>MSGSMKEEIKRLAEELKEKTKNEEIKRLAEEAAELAERSDDPEVLEVVKKALEEALKSKNEEKIELLLLVAVLVAEAGSVDAVEEKLEIALLALKLAEESKDPRIIRGALRAAIAALRSDDPLALKTVKEALERARASKDERLIRAILAAAYAFALLAVAGASAERLKEAEAIVKELIAAAEKGASPQELVLLVIEMMVKGMGVTMETHRSGNEVKVVIKGLHESQQEVLLEAVLFAAELMGVRVRIRFKGDTVTIVVREGSG[2x];>MSGEEAVRRRFEELLREALAFRERTGGRRETLEHAVRLARELAEFAASHPEFNRQEAVLLAIELMVRAMGVTMETHRSGNEVKVVIKGLNIDEQVALYRAVRETSKIMGVETEIEVEGDTQTIVVREGSG[2x]

Several natural systems exhibit ‘facilitated dissociation’, in which an effector (E) can bind to a target–host (TH) complex to form an excited ternary complex (THE)20–26 from which the target dissociates quickly. We set out to design protein systems that undergo facilitated dissociation. We use a switchable target binder (host) and a flexible effector that can rapidly bind to and switch the target–host complex to induce a large steric clash with the target, forming a strained excited ternary complex. We show here that by explicitly considering excited intermediate states when designing coupled protein systems, a broad range of facilitated dissociation systems can be designed.

We used X-ray crystallography to structurally characterize multiple states of our designed systems. The unbound structures show an open hydrophobic cleft in the new designed state X poised to bind the effector, and the effector-bound structures show that binding the effector causes the two switch domains to register-shift into the designed state Y. Structures of the target–AS1 complex show that the target binds as designed (top), with some strain suggested by small variations among the structures (bottom). For (1), the target dissociates 20-fold faster from AS1 than from an unhindered binder fusion, probably because of minor strain in the target–AS1 complex.> GPLGSQSHFIP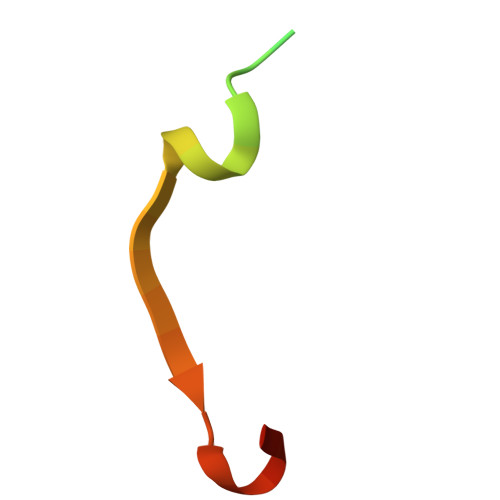ALFRPSPLERIKTNVINPAYATE> MFENITAAPADPILGLADLFRADERPGKINLGIGVYKDETGKTPVLTSVKKAEQYLLENETTKNYLGIDGIPEFGRCTQELL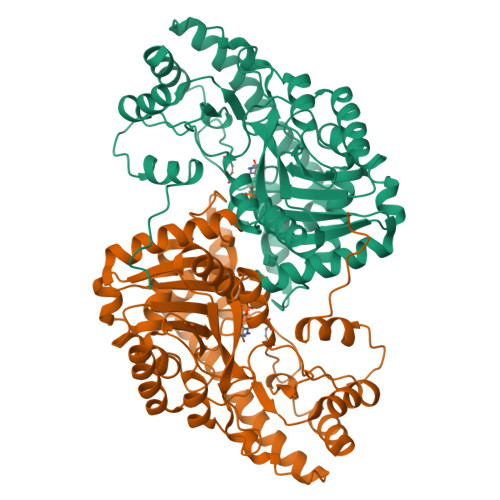FGKGSALINDKRARTAQTPGGTGALRVAADFLAKNTSVKRVWVSNPSWPNHKSVFNSAGLEVREYAYYDAENHTLDFDALINSLNEAQAGDVVLFHGFCHNPTGIDPTLEQWQTLAQLSVEKGWLPLFDFAYQGFARGLEEDAEGLRAFAAMHKELIVASSYSKNFGLYNERVGACTLVAADSETVDRAFSQMKAAIRANYSNPPAHGASVVATILSNDALRAIWEQELTDMRQRIQRMRQLFVNTLQEKGANRDFSFIIKQNGMFSFSGLTKEQVLRLREEFGVYAVASGRVNVAGMTPDNMAPLCEAIVAVL At the cytoplasmic face of the NPC, Nxf1•Nxt1-bound mRNPs encounter the cytoplasmic filament nucleoporins Gle1, Nup42, and Nup214, which specifically activate the DEAD-box helicase DDX19 to remove Nxf1•Nxt1 from the mRNP8. DDX19 is a member of the DEAD-box helicase family, which are RNA-dependent ATPases composed of two RecA domains (referred to as DDX19NTD and DDX19CTD throughout the text). Gle1CTD plays an important organizational role by providing spatially separated binding sites for Nup42GBM and the DEAD-box helicase DDX19/scDbp5. A comprehensive structure-function analysis of DDX19 indicates that binding of Gle1CTD•Nup42GBM induces a conformational change in DDX19, thereby stimulating its ATPase activity.

To understand the structural basis for IP6-independent DDX19 activation, we determined crystal structures of human Gle1CTD•Nup42GBM in complex with DDX19 in the presence of ADP or AMP-PNP•Mg2+ at 3.6 and 3.4 Å resolution, respectively. The heterotrimeric Gle1CTD•Nup42GBM•DDX19∆N53 complex exhibited similar conformations in the presence of ADP or AMP-PNP•Mg2+, with the auto-inhibitory helix still bound between DDX19NTD and DDX19CTD. The Gle1CTD−DDX19CTD interface involves 40 Gle1 and 35 DDX19 residues to generate an interaction interface area of almost 1300 Å2. In the first interface (interface 1), Gle1CTD residues of helix α4 (H495, E491, and Q487) form an extensive hydrogen bond network with each other and DDX19CTD main chain atoms (residues 380–382), as well as a salt bridge between Gle1CTD residue E491 and DDX19CTD residue K385. In the second interface (interface 2), the acidic C-terminal helix of DDX19CTD is recognized by lysines on the Gle1CTD surface, with salt bridges forming between DDX19CTD residues D470, D472, and E475 and Gle1CTD residues K416, K419, and K479. To gain further insight into how Gle1CTD•Nup42GBM binding facilitates DDX19 activation, we compared the structures of Gle1CTD•Nup42GBM•DDX19∆N53 to those of apo DDX19∆N53. The most apparent difference was a rotation of both DDX19NTD and the auto-inhibitory helix away from DDX19CTD, despite the auto-inhibitory helix still being bound between the two domains. Therefore, we considered our structure as an early intermediate state that forms immediately after Gle1CTD binding to DDX19, but before release of the auto-inhibitory helix and separation of DDX19NTD and DDX19CTD. In summary, Gle1CTD binding to DDX19CTD causes a cascade of conformational changes that partially releases the auto-inhibitory helix and prepares the residues involved in nucleotide binding to form the closed, active conformation.

>MQDITMQWYQQLQDASMQCVLTFEGLTNSKDSQAKKIKMDLQKAATIPVSQISTIAGSKLKEIFDKIHSLLSGKPVQSGGRSVSVTLNPQGLDFVQYKLAEKFVKQGEEEVASHHEAAFPIAVVASGIWELHPRVGDLILAHLHKKCPYSVPFYPTFKEGMALEDYQRMLGYQVKDSKVEQQDNFLKRMSGMIRLYAAIIQLRWPYGNRQEIHPHGLNHGWRWLAQILNMEPLSDVTATLLFDFLEVCGNALMKQYQVQFWKMLILIKEDYFPRIEAITSSGQMGSFIRLKQFLEKCLQHKDIPVPKGFLTSSFWRS[2x];>[2x]GPSGSIIATDNVLFTPRDKLTVEELEQFQSKKFTLGKIPLKPPPLELLNV;>GPHMEDRAAQSLLNKLIRSNLVDNTNQVEVLQRDPNSPLYSVKSFEELRLKPQLLQGVYAMGFNRPSKIQENALPLMLAEPPQNLIAQSQSGTGKTAAFVLAMLSQVEPANKYPQCLCLSPTYELALQTGKVIEQMGKFYPELKLAYAVRGNKLERGQKISEQIVIGTPGTVLDWCSKLKFIDPKKIKVFVLDEADVMIATQGHQDQSIRIQRMLPRNCQMLLFSATFEDSVWKFAQKVVPDPNVIKLKREEETLDTIKQYYVLCSSRDEKFQALCNLYGAITIAQAMIFCHTRKTASWLAAELSKEGHQVALLSGEMMVEQRAAVIERFREGKEKVLVTTNVCARGIDVEQVSVVINFDLPVDKDGNPDNETYLHRIGRTGRFGKRGLAVNMVDSKHSMNILNRIQEHFNKKIERLDTDDLDEIEKIAN[2x]>MESPSSEEEKPLAKMAFTLADRVTEEMLADKAALVVEVVEENYHDAPIVGIAVVNEHGRFFLRPETALADPQFVAWLGDETKKKSMFDSKRAAVALKWKGIELCGVSFDLLLAAYLLDPAQGVDDVAAAAKMKQYEAVRPDEAVYGKGAKRAVPDEPVLAEHLVRKAAAIWELERPFLDELRRNEQDRLLVELEQPLSSILAEMEFAGVKVDTKRLEQMGKELAEQLGTVEQRIYELAGQEFNINSPKQLGVILFEKLQLPVLKKTKTGYSTSADVLEKLAPYHEIVENILHYRQLGKLQSTYIEGLLKVVRPATKKVHTIFNQALTQTGRLSSTEPNLQNIPIRLEEGRKIRQAFVPSESDWLIFAADYSQIELRVLAHIAEDDNLMEAFRRDLDIHTKTAMDIFQVSEDEVTPNMRRQAKAVNYGIVYGISDYGLAQNLNISRKEAAEFIERYF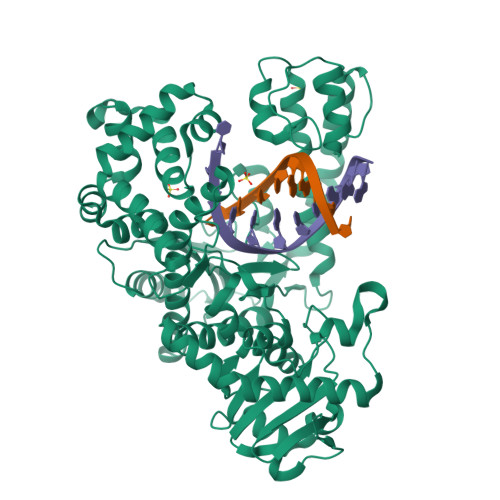ESFPGVKRYMENIVQEAKQKGYVTTLLHRRRYLPDITSRNFNVRSFAERMAMNTPIQGSAADIIKKAMIDLNARLKEERLQAHLLLQVHDELILEAPKEEMERLCRLVPEVMEQAVTLRVPLKVDYHYGSTWYDAK[2x]> MGSSHHHHHHSQGSMHYLDNLLLNTDSYKASHWLQYPPGTDASFFYVESRGGVYDQTAFFGLQSILKEAINRPVTHADIDDAKALLAAHGEPFNEAGWRDIVDRLGGQLPIRIRAVPEGCVVPTHNVLMTIESTDAKAFWVPSYLETLLLRVWYPVTVATVSWQVKQIVRDFLQRTSDDPEGQLPFKLHDFGARGVSSLGSAALGGAAHLVNFLGTDTLSALLLARAHYHTPVAGYSIPAAEHSTITSWGREREVDAYRNMLTQFARPGAIVAVVSDSYDIYRAIREHWGTTLREEIIASGATVVIRPDSGDPVDVVEQCLLLLDEAFGHQVNGKGYKVLNHVRVIQGDGINPQSLRAILERITAAGYAADNVAFGMGGALLQKVDRDTQKFALKCSAVRVDGAWIDVYKDPITDQGKQSKRGRLTLLRDRATGQYRSALLDEVATHAGDSDDALVTVWENGQMLREWTLEQVRAHADAARL

Nicotinamide phosphoribosyltransferase (NAMPT) plays an important role in the biosynthesis of nicotinamide adenine dinucleotide (NAD+) via the nicotinamide (NAM) salvage pathway. Here, we demonstrated the NAMPT-mediated salvage pathway is functional in the Gram-negative phytopathogenic bacterium Xanthomonas campestris pv. campestris (Xcc) for the synthesis of NAD+, and the enzyme activity of NAMPT in this bacterium is significantly higher than that of human NAMPT in vitro. Our structural analyses of Xcc NAMPT, both in isolation and in complex with either the substrate NAM or the product nicotinamide mononucleotide (NMN), uncovered significant details of substrate recognition. Specifically, we revealed the presence of a NAM binding tunnel that connects the active site, and this tunnel is essential for both catalysis and inhibitor binding.

We obtained two apo structures from two types of crystals, namely the tablet-shaped (1.79 Å) and diamond-shaped (2.08 Å) crystals. These structures had almost identical overall conformations (RMSD, 0.3 Å). However, since the structure determined from the diamond-shaped crystal was incomplete in domain A, we focused on describing the more complete apo structure obtained from the tablet-shaped crystal.>GSHMQTLLALNWKMNKTPTEARSWAEELTTKYAPAEGVDLAVLAPALDLSALAANLPAGIAFGGQDVSAHESGAYTGEISAAMLKDAGASCVVVGHSERREYHDESDATVAAKARQAQANGLLPIVCVGENLDVRERGEHVPQTLAQLRGSLEGVGADVVVAYEPVWAIGTGKTATADDAEELAAAIRGALREQYGARAEGIRVLYGGSVK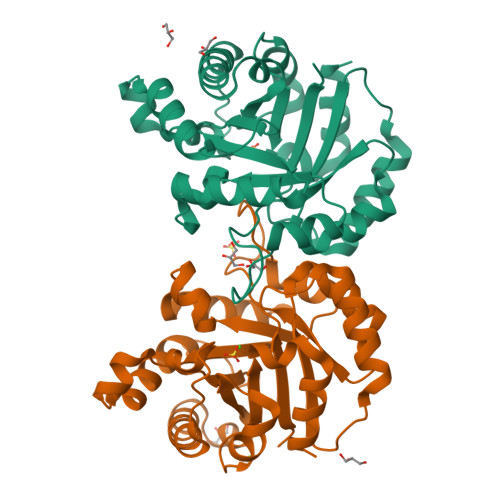PENIAEICGKPNVNGALVGGASLKVPDVLGMLDALR[4x]> PHLRTFKDNFQTCKVEGAWPLIDNNYLSVQVTNVPVVPGSSATATNKITIIFKAHHGCTDQKVYQAVTDDLPAAFVDGTTSGGDSDAKSLRIVERESGHYVEMHARYIGTTV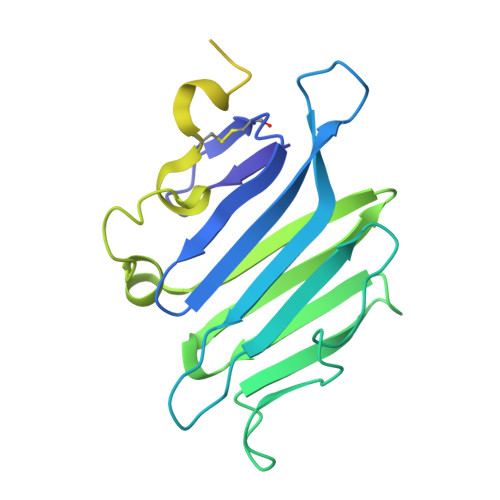FVRQVGRYLTLAIRMPEDLAMSYEESQDLQLCVNGCPLSERIDDGQGQVSAILGHSLPRTSLVQAWPGYTLETANTQCHEKMPVKDIYFQSCVFDLLTTGDANFTAAAHSALEDVEALHPRKERWHIFPSGTKHHHHHH>MNDKKIELLTTYLSLYIDHHTVLADMQNATGKYVVLDVRNAPAQVKKDQIKGAIAMPAKDLATRIGELDPAKTYVVYDWTGGTTLGKTALLVLLSAGFEAYELAGAL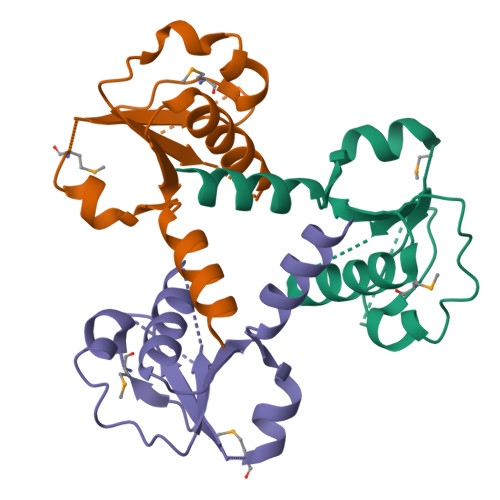EGWKG[6x]>MNSENTIVYVRVAGRARNGFVDPLKFYWDLERDRSLWSSVSKLDNTKKTIDWKRLSREFKAPEHFIRKRSYALFAKHLKLLERQIEA[2x];>[2x]MSSEANPPVLEPFTVTVVDRNVKHQVEGEPEEEGHPDHEVQGVMFATNVKYIFEDDQELLPEQEDPAIENVVIIEADESLRVTQVELISDQFKQVGYEVRDGNEVCIDALSRFETPRQLGNLPLEKLVQLYKLQNDQLHSLFNTLHHHHHH;>MNEAVIEKLLENSRKFLTGAKLICQESNDHLTTTKLRIREWQKFQSKLHFVLDCIQQQTKFLSEILLREGIGRNLIEEEWSQTVLVRLVND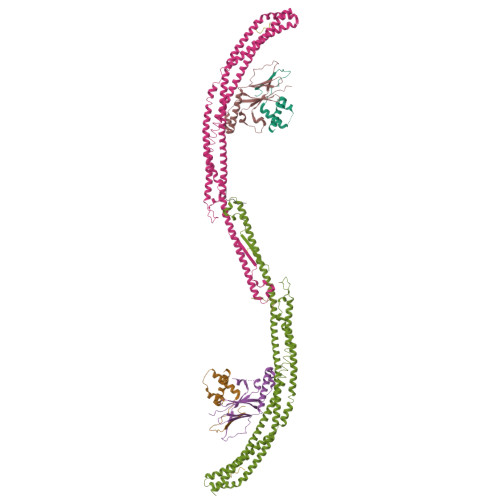MKFWQNEITKMMNKLDNITNEIDQQHNSKLGDFISRDSSHILDSKLNEIPTIRKQVENITRQYQTMLAKVQSQLVESRMKGLRDEFSSKFGDQCRENLKLNEEFTNEADQLEQELADFLKSFTDHFDKCSALSSRSVSPEDAQNLFEIVERDDKDLAAINSLLQDAAIDVASFVRKVNMLLDERDADKAKMQATLSKLLTELRKHEEYISVFEGISALIQKFKASCLEDIRQTRNLLDFYANFERSYHNLLKEVKRRKETAAKLSQILKSCETQLEQINTADLRERQMFLLENGNYLPETIWPDEIGSLSPLYTLNYEVRKV[2x];>SKYSSSFGRLRRQ[2x];>[2x]LQPFKAGSVGSGS> MDKFRVQGPTRLQGEVTISGAKNAALPILFAALLAEEPVEIQNVPKLKDIDTTMKLLTQLGTKVERDGSVWIDASNVNNFSAPYDLVKTMRASIWALGPLVARFGQGQVSLPGGCAIGARPVDLHIFGLEKLGAEIKLEEGYVKASVNGRLKGAHIVMDKVSVGATVTIMSAATLA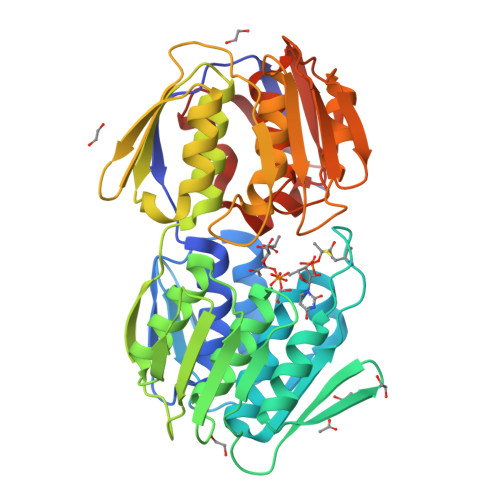EGTTIIENAAREPEIVDTANFLVALGAKISGQGTDRITIEGVERLGGGVYRVLPDRIETGTFLVAAAISGGKIVCRNAQPDTLDAVLAKLREAGADIETGEDWISLDMHGKRPKAVTVRTAPHPAFPTDMQAQFTLLNLVAEGTGVITETIFENRFMHVPELIRMGAHAEIESNTVICHGVEKLSGAQVMATDLRASASLVLAGCIAEGTTVVDRIYHIDRGYERIEDKLRALGANIERVKGE>MTPEAAYQNLLEFQRETAYLASLGALAAWDQRTMIPKKGHEHRARQMAALARLLHQRMTDPRIGEWLEKVEGSPLVQDPLSDAAVNVREWRQAYERARAIPERLAVELAQAESEAESFWEEARPRDDWRGFLPYLKRVYALTKEKAEVLFALPPAPGDPPYGELYDALLDGYEPGMRARELLPLFAELKEGLKGLLDRILGSGKRPDTSILHRPYPVEAQRRFALELLSACGYDLEAGRLDPTAHPFEIAIGPGDVRITTRYYEDFFNAGIFGTLHEMGHALYEQGLPKEHWGTPRGDAVSLGVHESQSRTW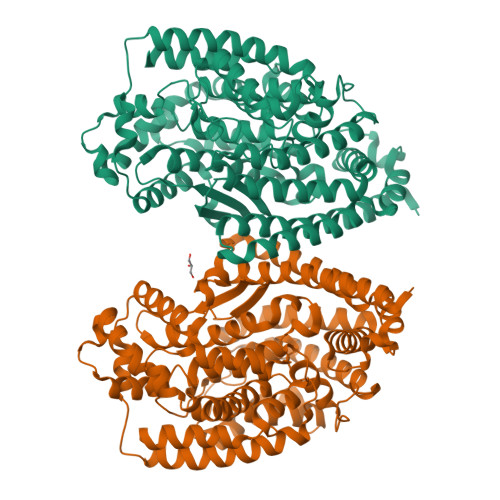ENLVGRSLGFWERFFPRAREVFASLGDVSLEDFHFAVNAVEPSLIRVEADEVTYNLHILVRLELELALFRGELSPEDLPEAWAEKYRDHLGVAPKDYKDGVMQDVHWAGGLFGYFPTYTLGNLYAAQFFQKAEAELGPLEPRFARGEFQPFLDWTRARIHAEGSRFRPRVLVERVTGEAPSARPFLAYLEKKYAALY[2x]>MNELPGTSDTPLLDQIHGPKDLKRLSREQLPALTEELRGEIVRVCSRGGLHLASSLGAVDIITALHYVLDSPRDRILFDVGHQAYAHKILTGRRDQMADIKKEGGISGFTKVSESEHDAITVGHASTSLTNALGMALARDAQGKDFHVAAVIGDGSLTGGMALAALNTIGDMGRKMLIVLNDNEMSISENVGAMNKFMRGLQVQKWFQEGEGAGKKAVEAVSKPLADFMSRAKNSTRHFFDPASVNPFAAMGVRYVGPVDGHNVQELVWLLERLVDLDGPTILHIVTTKGKGLSYAEADPIYWHGPAKFDPATGEYVPSSAYSWSAAFGEAVTEWAKTDPRTFVVTPAMREGSGLVEFSRVHPHRYLDVGIAEEVAVTTAAGMALQGMRPVVAIYSTFLQRAYDQVLHDVAIEHLNVTFCIDRAGIVGADGATHNGVFDLSFLRSIPGVRIGLPKDAAELRGMLKYAQTHDGPFAIRYPRGNTAQVPAGTWPDLKWGEWERLKGGDDVVILAGGKALDYALKAAEDLPGVGVVNARFVKPLDEEMLREVGGRARALITVEDNTVVGGFGGAVLEALNSMNLHPTVRVLG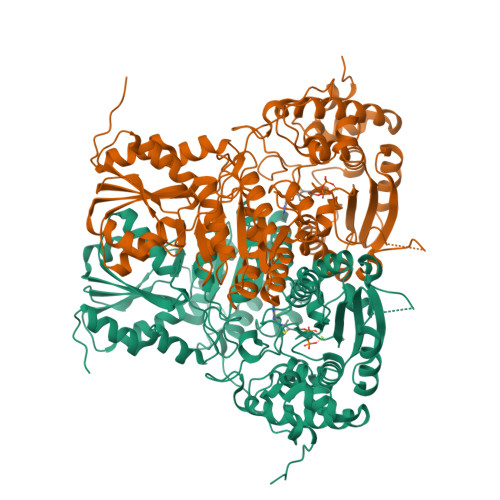IPDEFQEHATAESVHARAGIDAPAIRTVLAELGVDVPIEV[4x]> MAAAAGSCARVAAWGGKLRRGLAVSRQAVRSPGPLAAAVAGAALAGAGAAWHHSRVSVAARDG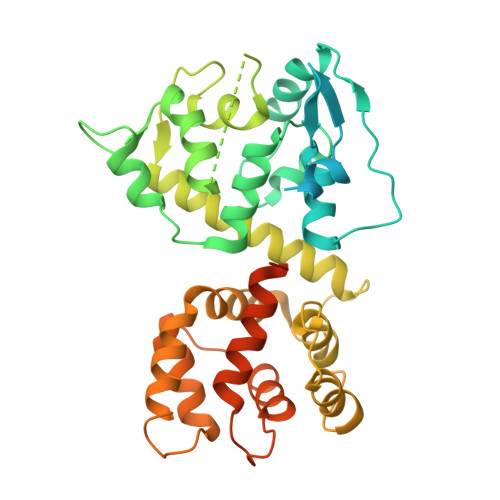SFTVSAQKNVEHGIIYIGKPSLRKQRFMQFSSLEHEGEYYMTPRDFLFSVMFEQMERKTSVKKLTKKDIEDTLSGIQTAGCGSTFFRDLGDKGLISYTEYLFLLTILTKPHSGFHVAFKMLDTDGNEMIEKREFFKLQKIISKQDDLMTVKTNETGYQEAIVKEPEINTTLQMRFFGKRGQRKLHYKEFRRFMENLQTEIQEMEFLQFSKGLSFMRKEDFAEWLLFFTNTENKDIYWKNVREKLSAGESISLDEFKSFCHFTTHLEDFAIAMQMFSLAHRPVRLAEFKRAVKVATGQELSNNILDTVFKIFDLDGDECLSHEEFLGVLKNRMHRGLWVPQHQSIQEYWKCVKKESIKGVKEVWKQAGKGLF>HTDLSGKVFVFPRESVTDHVNLITPLEKPLQNFTLCFRAYSDLSRAYSLFSYNTQGRDNELLVYKERVGEYSLYIGRHKVTSKVIEKFPAPVHICVSWESSSGIAEFWINGTPLVKKGLRQGYFVEAQPKIVLGQEQDSYGGKFDRSQSFVGEIGDLYMWDSVLPPENILSAYQGTPLPANILDW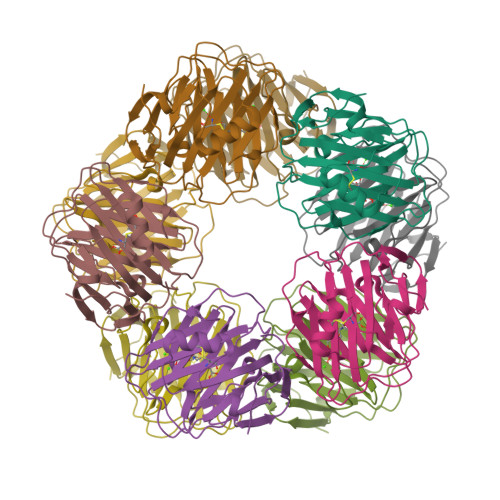QALNYEIRGYVIIKPLVWV[20x]A central regulatory mechanism of iron homeostasis in humans involves ferroportin (FPN), the sole cellular iron exporter, and the peptide hormone hepcidin, which inhibits Fe2+ transport and induces internalization and degradation of FPN. Vamifeport competes with hepcidin for FPN binding and is currently in clinical development for β-thalassemia and sickle cell disease. Here, we describe the cryo-electron microscopy structures of human FPN in complex with synthetic nanobodies and vamifeport (VIT-2763), the first clinical-stage oral FPN inhibitor. The structures display two distinct conformations of FPN, representing outward-facing and occluded states of the transporter.

Whereas, the hsFPN/Sy12/vamifeport complex shows an outward-facing conformation in the absence of bound metal ions that closely resembles equivalent states determined in previous studies, two hsFPN/Sy3 structures obtained in the absence and presence of vamifeport display a previously unknown conformation of FPN, where the access to substrate binding sites from the outside has closed, while the intracellular part of the transporter has remained unchanged. In contrast, the quality of the map of the hsFPN/Sy12/vamifeport complex is to some degree compromised by a preferential orientation of the particles and difficulties to reconstruct and refine a 3D model as a consequence of the binding of Sy12 to a flexible loop region at the periphery of the protein. Still, even in latter case, the map was sufficiently well resolved to permit its interpretation by an atomic model for the bulk of the transporter (Figure 2—figure supplements 1 and 4). Although the cryo-EM density of Sy12 is insufficiently well defined for a detailed interpretation, it permitted the placement of a model consisting of the conserved part of the binder as rigid unit. In this position, the interaction with the extracellular loop connecting α3 and α4 located at the periphery of the N-domain is apparent. Notably, the same loop is recognized by Fab45D8, which was used to determine hsFPN structures in a previous study (Billesbølle et al., 2020). In the hsFPN/Sy3 map obtained from a sample containing vamifeport, we noticed a pronounced elongated density of appropriate size and shape of the inhibitor that is not present in a structure of the same protein complex obtained in its absence, where also the proximal α7a–α7b loop appears more mobile. Residual density at an equivalent location is also observed in the outward-facing structure of the hsFPN/Sy12 complex obtained in the presence of vamifeport. However, the density is, in this case, less well defined, which likely reflects a preferred binding of the molecule to the occluded state, although it might in part also be a consequence of the lower resolution of the map and the compromised quality resulting from the described preferential orientation of particles.

> MSTRAGDHNRQRGCCGSLADYLTSAKFLLYLGHSLSTWGDRMWHFAVSVFLVELYGNSLLLTAVYGLVVAGSVLVLGAIIGDWVDKNARLKVAQTSLVVQNVSVILCGIILMMVFLHKHELLTMYHGWVLTSCYILIITIANIANLASTATAITIQRDWIVVVAGEDRSKLANMNATIRRIDQLTNILAPMAVGQIMTFGSPVIGCGFISGWNLVSMCVEYVLLWKVYQKTPALAVKAGLKEEETELKQLNLHKDTEPKPLEGTHLMGVKDSNIHELEHEQEPTCASQMAEPFRTFRDGWVSYYNQPVFLAGMGLAFLYMTVLGFDCITTGYAYTQGLSGSILSILMGASAITGIMGTVAFTWLRRKCGLVRTGLISGLAQLSCLILCVISVFMPGSPLDLSVSPFEDIRSRFIQGESITPTKIPEITTEIYMSNGSNSANIVPETSPESVPIISVSLLFAGVIAARIGLWSFDLTVTQLLQENVIESERGIINGVQNSMNYLLDLLHFIMVILAPNPEAFGLLVLISVSFVAMGHIMYFRFAQNTLGNKLFACGPDAKEVRKENQANTSVVALEVLFQG>[2x]SKPQPIAAANWKSGSPDSLSELIDLFNSTSINHDVQCVVASTFVHLAMTKERLS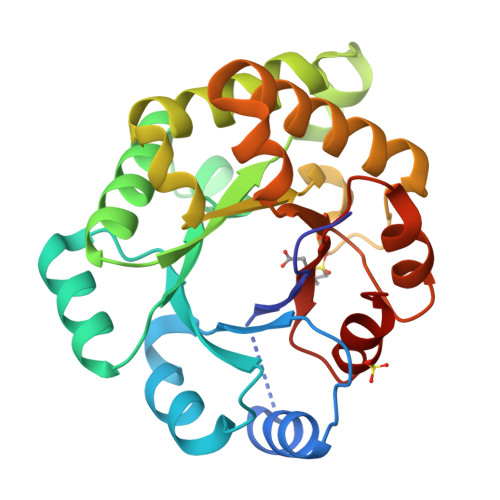HPKFVIAAQNAGNADALASLKDFGVNWIVLGHSERRWYYGETNEIVADKVAAAVASGFMVIACIGETLQERESGRTAVVVLTQIAAIAKKLKKADWAKVVIAYEPVWAIGTGKVATPQQAQEAHALIRSWVSSKIGADVAGELRILYGGSVNGKNARTLYQQRDVNGFLAGLKPEFVDIIKATQ>[2x]MREMHHSRWSKIGTALAVSSALGLMSGMSVANDKLVELSKSNENWVMQGKDFSGTHYSTAKQINKDNVKKLRPSWSFSTGVLNGHEGAPLVVNGTMYIHTPFPNNTFAIDLDEPGVIKWEHKPKQDPAARAVACCDVVNRGLAYWPGDDKAPAMIVKSLLDGHVVALNAETGEEYWKVENGDISVGQTETAAPFVAKDLVIQGSSGAELGVRGYVTAYDIHTGEMVWRWYATGPDADVGLDKDFNKHNPHYGQKGLGTSTWEDNAWKIGGGTNWGWYAYDPQLDMFYYGSGNPAPWNETMRPGDNKWTMTIWGRDLETGLAKFGYQKTPHDEWDYAGVNVMMLSEQKDKNGKMRKLLTHPDRNGIIYTLDRETGDLVSANKMDDTANWVKKVDLETGLPIRDP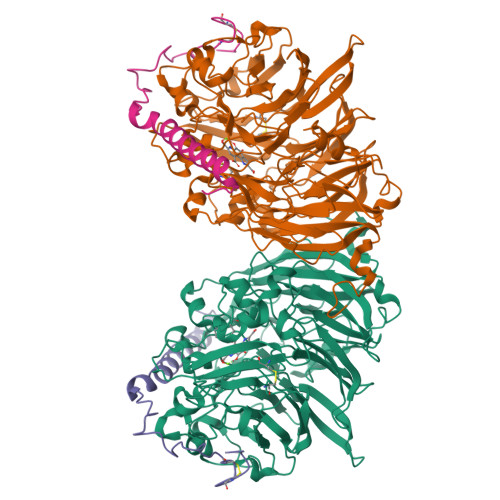EYGTRMGHRSRDVCPSAMGFHNQGFDSYDPKRELFYLGINHLCMDWEPFMLPYRAGQFFVGANVWTYPGPKGDRQNGIGSGQVKAYNAITGEFAWEKMEKFSVWGGTTATEGGLVFYGTLDGFIKARDADTGKLLWKFKLPSGVIGHPMTYTHKGTQYVAINYGVGGWPAVGLVFDLNDPSAGLGAVGAFKELAKNTQMGGGVMVFSLDGKSPYDDVSLGEYGM;>MKLKTIAVACSALMMLSGASAVMAYDGTKCKAAGDCWEAKPGFPDKIKGSKYDPKHSEKELNKQDAALKAMEKRNAERVEQFKKTGKWVY[2x]>[2x]MVVSIGVFDGVHIGHQKVLRTMKEIAFFRKDDSLIYTISYPPEYFLPDFPGLLMTVESRVEMLSRYARTVVLDFFRIKDLTPEGFVERYLSGVSAVVVGRDFRFGKNASGNASFLRKKGVEVYEIEDVVVQG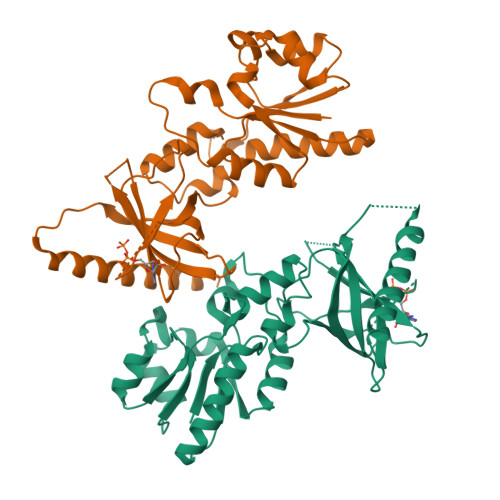KRVSSSLIRNLVQEGRVEEIPAYLGRYFEIEGIVHKDREFGRKLGFPTANIDRGNEKLVDLKRGVYLVRVHLPDGKKKFGVMNVGFRPTVGDARNVKYEVYILDFEGDLYGQRLKLEVLKFMRDEKKFDSIEELKAAIDQDVKSARNMIDDIINSKFEKEG> MMFGRFTERAQKVLALAQEEALRLGHNNIGTEHILLGLVREGEGIAAKALQAL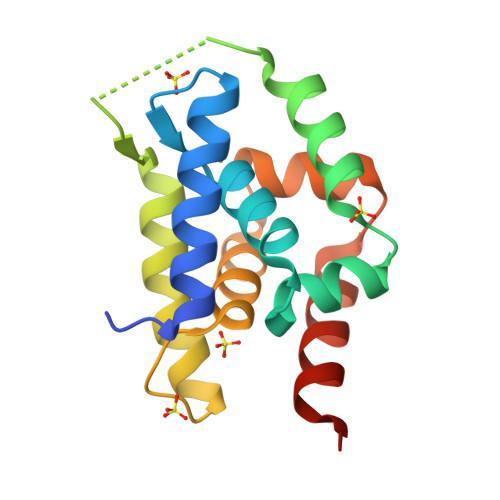GLGSEKIQKEVESLIGRAQEMSQTIHYTPRAKKVIELSMDEARKLGHSYVGTEHILLGLIREGEGVAARVLNNLGVSLNKARQQVLQLLGNNETGSS> VRLGSML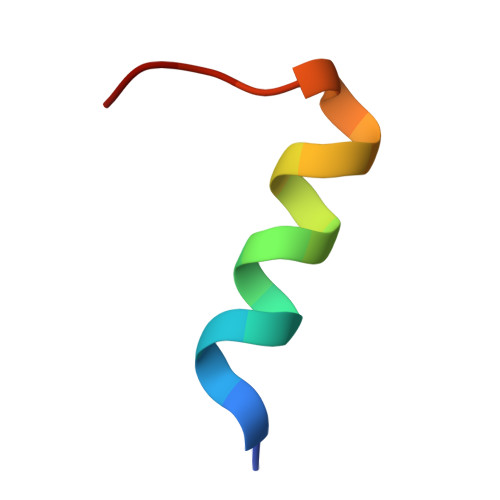ASIGQEIGGVEL> GSHMASSCAVQVKLELGHRAQVRKKPTVEGFTHDWMVFVRGPEHSNIQHFVEKVVFHLHESFPRPKRVCKDPPYKVEESGY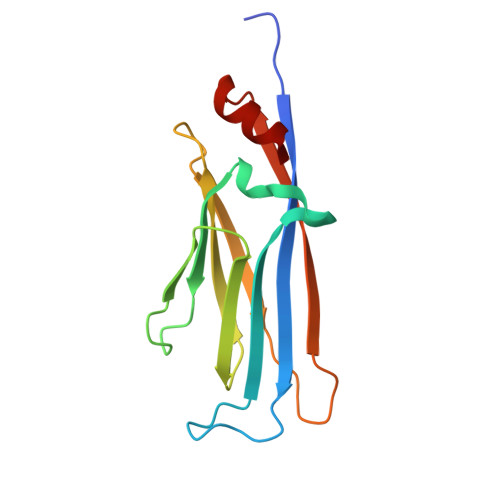AGFILPIEVYFKNKEEPRKVRFDYDLFLHLEGHPPVNHLRCEKLTFNNPTEDFRRKLLKA> MNQNLLVTKRDGSTERINLDKIHRVLDWAAEGLHNVSISQVELRSHIQFYDGIKTSDIHETIIKAAADLISRDAPDYQYLAARLAIFHLRKKAYGQFEPPALYDHVVKMVEMGKYDNHLLEDYTEEEFKQMDTFIDHDRDMTFSYAAVKQLEGKYLVQNRVTGEIYESAQFLYILVAACLFSNYPRETRLQYVKRFYDAVSTFKISLPTPIMSGVRTPTRQFSSCVLIECGDSLDSINATSSAIVKYVSQRAGIGINAGRIRALGSPIRGGEAFHTGCIPFYKHFQTAVKSCSQGGVRGGAATLFYPMWHLEVESLL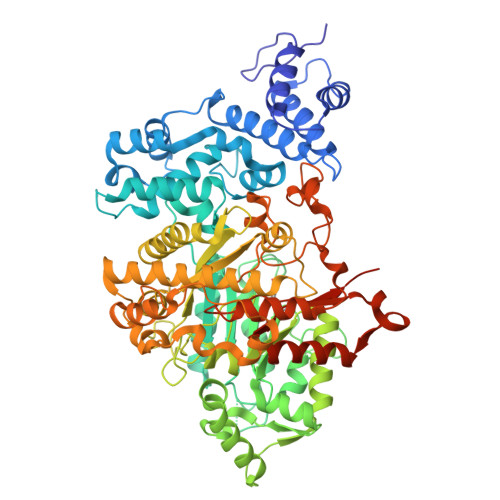VLKNNRGVEGNRVRHMDYGVQINKLMYTRLLKGEDITLFSPSDVPGLYDAFFADQEEFERLYTKYEKDDSIRKQRVKAVELFSLMMQERASTGRIYIQNVDHCNTHSPFDPAIAPVRQSNLCLEIALPTKPLNDVNDENGEIALCTLSAFNLGAINNLDELEELAILAVRALDALLDYQDYPIPAAKRGAMGRRTLGIGVINFAYYLAKHGKRYSDGSANNLTHKTFEAIQYYLLKASNELAKEQGACPWFNETTYAKGILPIDTYKKDLDTIANEPLHYDWEALRESIKTHGLRNSTLSALMPSETSSQISNATNGIEPPRGYVSIKASKDGILRQVVPDYEHLHDAYELLWEMPGNDGYLQLVGIMQKFIDQSISANTNYDPSRFPSGKVPMQQLLKDLLTAYKFGVKTLYAQNTRDGAEDAQDDLVPSIQDDGCESGACKI Toll-like Receptor 3 (TLR3) plays a key role in anti-viral defenses by inducing a potent immune response against double-stranded RNAs (dsRNAs) produced by viral infection. Previous crystallographic studies show that RNA ligand binds to the extracellular domains of TLR3 and induces the formation of a homodimer of TLR326. The charge interaction with the phosphate backbone of the RNA double helix plays the principal role in the interaction. The ligand-binding site involves both the N and C-terminal parts of the TLR3 ectodomain.

To determine the structure of the TLR3-dsRNA complex, we mixed purified full-length TLR3 with a poly(I:C) dsRNA. The length of the poly(I:C) used in the experiments ranged from 200 bp to 1,500 bp, with an average length of ~400 bp. The raw micrographs showed that a vast majority of TLRs are linearly assembled along the RNA strands with regular spacing. The final reconstituted three-dimensional structure shows a 2.8 Å resolution image of the TLR3 tetramers on the RNA strands. The cryo-EM map resolution was estimated to be 2.8 Å, but the RNA region between the TLR3 dimeric units has structural flexibility that prohibited refinement to a higher resolution. However, when the refinement was focused on the dimeric area of the cluster, a 2.3 Å resolution could be achieved. In the structure, the RNA double helix is bent by ~8 degrees at the junction between the two TLR3 dimeric units. Our cryo-EM structure of TLR3 is practically identical to the reported crystal structure with a Cα root mean square deviation (r.m.s.d.) of 0.77 Å. This result demonstrates that linear clustering does not disturb the structure of the dimeric unit of the TLR3-dsRNA complex. The dimeric units of TLR3 are repeated 2~20 times with a regular spacing of 103 Å or 34 RNA base pairs in the cluster.

>STTKCTVSHEVADCSHLKLTQVPDDLPTNITVLNLTHNQLRRLPAANFTRYSQLTSLDVGFNTISKLEPELCQKLPMLKVLNLQHNELSQLSDKTFAFCTNLTELHLMSNSIQKIKNNPFVKQKNLITLDLSHNGLSSTKLGTQVQLENLQELLLSNNKIQALKSEELDIFANSSLKKLELSSNQIKEFSPGCFHAIGRLFGLFLNNVQLGPSLTEKLCLELANTSIRNLSLSNSQLSTTSNTTFLGLKWTNLTMLDLSYNNLNVVGNDSFAWLPQLEYFFLEYNNIQHLFSHSLHGLFNVRYLNLKRSFTKQSISLASLPKIDDFSFQWLKCLEHLNMEDNDIPGIKSNMFTGLINLKYLSLSNSFTSLRTLTNETFVSLAHSPLHILNLTKNKISKIESDAFSWLGHLEVLDLGLNEIGQELTGQEWRGLENIFEIYLSYNKYLQLTRNSFALVPSLQRLMLRRVALKNVDSSPSPFQPLRNLTILDLSNNNIANINDDMLEGLEKLEILDLQHNNLARLWKHANPGGPIYFLKGLSHLHILNLESNGFDEIPVEVFKDLFELKIIDLGLNNLNTLPASVFNNQVSLKSLNLQKNLITSVEKKVFGPAFRNLTELDMRFNPFDCTCESIAWFVNWINETHTNIPELSSHYLCNTPPHYHGFPVRLFDTSSCKDSAPFELFFMINTSILLIFIFIVLLIHFEGWRISFYWNVSVHRVLGFKEIDRQTEQFEYAAYIIHAYKDKDWVWEHFSSMEKEDQSLKFCLEERDFEAGVFELEAIVNSIKRSRKIIFVITHHLLKDPLCKRFKVHHAVQQAIEQNLDSIILVFLEEIPDYKLNHALCLRRGMFKSHCILNWPVQKERIGAFRHKLQVALGSKNSVHSNSLEVLFQ[4x]>[2x]LGRHFYVTGPVVRGAGRGGKELGFPTANQYFHDTVALPADGVYAGWLTILPTEAPVSGNMEPEVAYAAAISVGTNPTFGD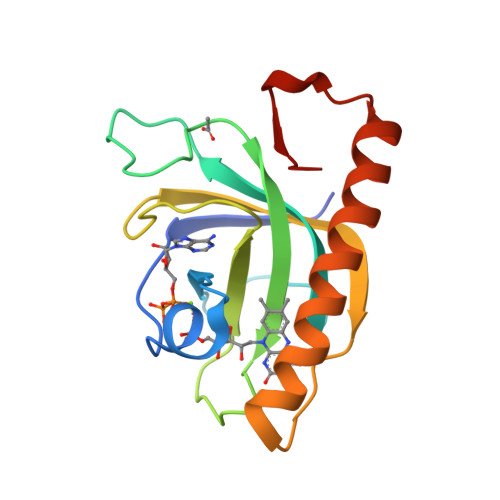EQRSVESFVLDRDADLYGHDVKVEFVDHVRAMEKFDSVEQLLEVMAKDVQKTRTLLAQDVQAHKMAPETYFLQAES> PIFLNVLEAIEPGVVCAGHDNNQPDSFAALLSSLNELGERQLVHVVKWAKALPGFRNLHVDDQMAVIQYSWMGLMVFAMGWRSFTNVNSRMLYFAPDLVFNEYRMHKSRMYSQCVRMRHLSQEFGWLEITPQEFLCMKALLLFSIIPVDGLKNQKFFDELRMNYIKELDRIIACKRKNPTSCSRRFYQLTKLLDSVQPIARELHQFTFDLLIKSHMVS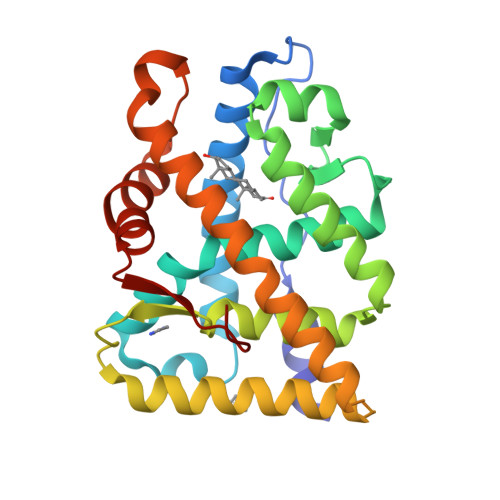VDFPEMMAEIISVQVPKILSGKVKPIYFHTQ>GRPFVEMYSEIPEIIHMTEGRELVIPCRVTSPNITVTLKKFPLDTLIPDGKRIIWDSRKGFIISNATYKEIGLLTCEATVNGHLYKTNYLTHRQ[4x]

Three receptor types have been highlighted: VEGFR3 (also called Flt-4) regulates lymphangiogenesis, VEGFR2 (KDR/Flk-1) is the primary proangiogenic receptor, whereas VEGFR1 (Flt-1) has been proposed as a regulator of VEGFR2. In this study, we showed the presence of a metal site at the dimer interface of X-ray structures of human VEGFR1 domain 2 (hVEGFR1d2) solved in the presence of different divalent metal ions. The three structures are similar and reveal a homodimer with interlocked hydrophobic surfaces buried at the interface and a divalent cation chelated by four histidine residues (two from each monomer). Importantly, the dimer interface involves residues that lie in the core of the hVEGFR1d2 surface that interacts with VEGF-A, VEGF-B or PlGF.

The structures of the P1, C2221 and I222 crystal forms were determined with four molecules, one molecule and three molecules in the asymmetric unit respectively. The Co2+ ion was coordinated through the Nε atoms of the imidazole groups of His147 and His223 on each domain and by two water molecules to form a square-based bipyramidal regular octahedron. Three additional Co2+ ions, which exhibited higher B factors, were present in the asymmetric unit and were also coordinated by a histidine residue (His214). The metal ion coordination site is octahedral for Co2+ and tetrahedral for Zn2+ and Cu2+. Superposition of one hVEGFR1d2 molecule of the Co2+-bound and Zn2+- or Cu2+-bound dimers resulted in a maximum rotation for the second molecule by 12° and a translation of 2.4 Å. The mean estimation for ΔG dissociation was 12.7 kcal.mol-1, 58.1 kcal.mol-1 and 18.4 kcal.mol-1 for (hVEGFR1d2)2-Co2+, -Zn2+, and -Cu2+ respectively. To verify that the homodimer observed in the crystal forms existed in solution, we performed SAXS analysis of hVEGFR1d2 in the presence of 10 mM CoCl2 or after thorough removal of all traces of divalent cations. The SAXS results unambiguously indicated that 10 mM Co2+ induced a doubling of the molecular weight and a significant increase of the radius of gyration, confirming the Co2+-induced dimerization of the hVEGFR1d2 domain in solution. Theoretical data calculated by CRYSOL fitted well with data measured in the presence of Co2+ (hVEGFR1d2 dimer crystal structure) or in the absence of Co2+ (hVEGFR1d2 monomer structure). Other divalent cations exhibited little (Co2+ and Cd2+) or no effect on the competition assay (Fe2+ and Mn2+).> MSFRFGQHLIKPSVVFLKTELSFALVNRKPVVPGHVLVCPLRPVERFHDLRPDEVADLFQTTQRVGTVVEK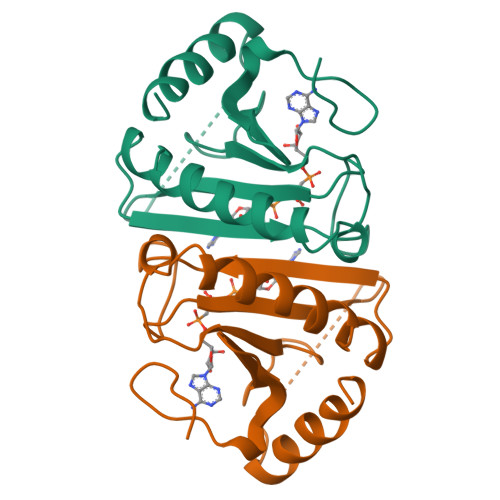HFHGTSLTFSMQDGPEAGQTVKHVHVHVLPRKAGDFHRNDSIYEELQKHDKEDFPASWRSEEEMAAEAAALRVYFQ>[2x]MRNDGGFLDWWEDLRSEMQSITDSQEVFAVLEKEVRRLGFDYYAYCVRHPIPFTRPRIFMF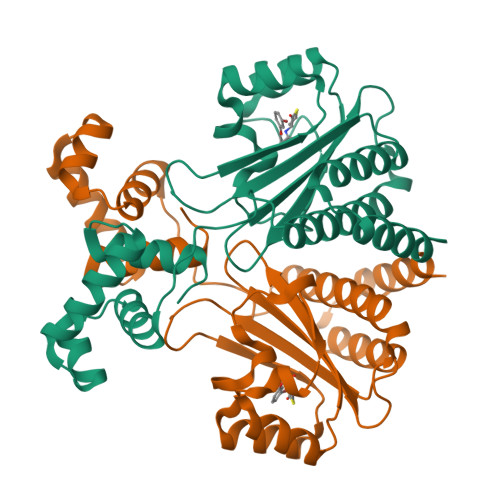GNYPPAWQEHYQAQNYFAIDPTIRHCLRSGNHIVWSDDLFADAQELWDDARDYGLRHGATHSCMAPNGVMGFLSVARSSPAISPHEREELRLRMRCLIELLHQTLTELNHPSLQPQPICLSKREREILRWTADGKTSAEIAKILGISESTVNFHLKNIQKKFNAPNKTQAAAYAAALGLI>[4x]MSGFSTEERAAPFSLEYRVFLKNEKGQYISPFHDIPIYADKDVFHMVVEVPRWSNAKMEIATKDPLNPIKQDVKKGKLRYVANLFPYKGYIWNYGAIPQTWEDPGHNDKHTGCCGDNDPIDVCEIGSKVCARGEIIGVKVLGILAMIDEGETDWKVIAINVDDPDAANYNDINDVKRLKPGYLEATVDWFRRYKV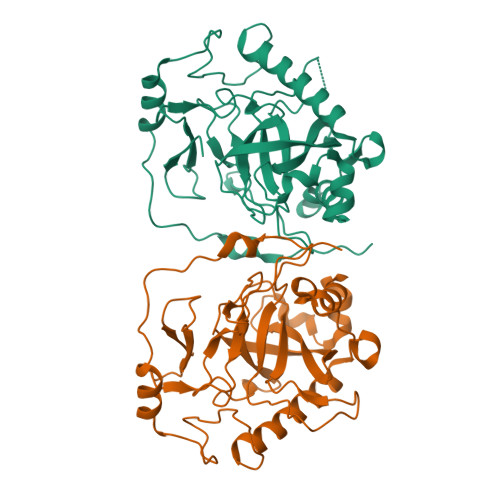PDGKPENEFAFNAEFKDKDFAIDIIKSTHDHWKALVTKKTNGKGISCMNTTLSESPFKCDPDAARAIVDALPPPCESACTVPTDVDKWFHHQKN> MRGSHHHHHHTDPQGDAAQKTDTSHHDQDHPTFNKITPNLAEFAFSLYRQLAHQSNSTNIFFSPVSIATAFAMLSLGTKADTHDEILEGLNFNLTEIPEAQIHEGFQELLRTLNQPDSQLQLTTGNGLFLSEGLKLVDKFLEDVKKLY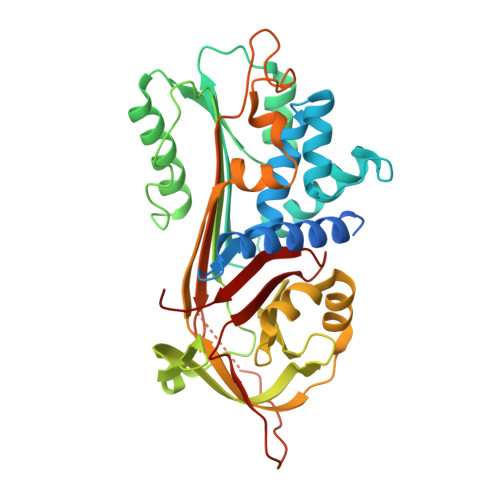HSEAFTVNFGDTEEAKKQINDYVEKGTQGKIVDLVKELDRDTVFALVNYIFFKGKWERPFEVKDTEEEDFHVDQVTTVKVPMMKRLGMFNIQHCKKLSSWVLLMKYLGNATAIFFLPDEGKLQHLENELTHDIITKFLENEDRRSASLHLPKLSITGTYDLKSVLGQLGITKVFSNGADLSGVTEEAPLKLSKAVHKAVLTIDEKGTEAAGAMFLEAIPMSIPPEVKFNKPFVFLFIEQNTKSPLFMGKVVNPTQK>[2x]GQPTGTMTTDSKLTSKESALALTNSAYLKNTVFNKMTPGWGCNTILLLEYMTGKATSENSQSNYKDFQDLLVSDRSLYIEDWWQDCYAGIANCNLALQKLGEFENLDASLVNGYMAEVKFMRALYYFYLVRIFGDVPKITTVQSELGELQVSRAPVKEIYDEIIIPDLLEAEQSD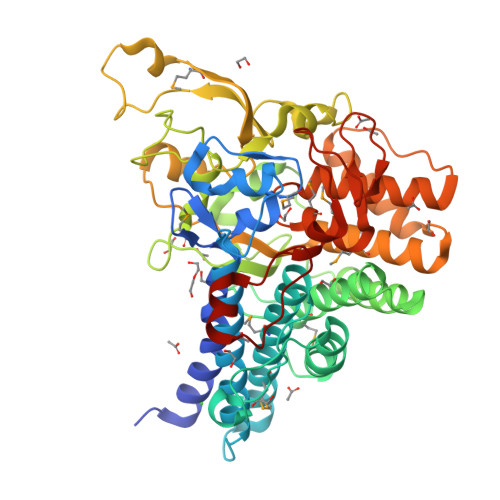LAFSDHTGRVSMGAVKALLADVYLTYAGYPLQGGKSYYAESAKRSLEVIKSNEYTLFTDYESLRLPSQNNKGEFIYQVQFSLNKRHNESVRIFLPSRSGISAYDLEYGSLIPTKEFVESFEKGDKRTEEKQYFFTNYKGHPSKFSPGAAELEFMDLNGYYIYKFFDQVAVDNTAKSDLNWSVYRYTDVLLMYAEAQVNADGTPNQQSIDIVNQIRGRAGLAPFKQTNASAFLEEVWDQRYFDLCYENKMWFDMLRTRKIRDDKSGEYVDFIGYKTNWGKVYTETQLLFPIPLSERQANPNLTQNQGY> GMSEPYTWKSVVTGAGGGFVPGIIFNQTEPNLIYARTAIGGAYRWNQATSSWVSISDSVGWVDWNKNGVDALATDPIDPNKVYMATGTYTNHWDNNGQIMRSNDRGNTWQTTPLPFKVGGNMPGRSAGERLVIDPNKNNILYFGARSGNGLWKSIDSGVTWSKVTSFPNVGTYIQNPTLDYGNDLVGLSWITFDKSTGTLGNATQTIYVGVADTASSVYRSTDGGVTWTALAGQPTGFLPHHGELSSTGDLYITYSNGVGPYDGSKGEVWKYNKTSGAWTNISPTTGTDNWYGFGGLALDAQHPNTLMVSSLNAWWPDEVIFRSTNGGATWSRIWDWGNYPERTYKFSMDITAAPWLDHGTTSTSLDPSPKLGWMMGDLEIDPFNSNRMMYGTGATIYGSNNLTSWDTGGKVNISVMAKGVEETAVLGLISPPTGTSHLITALGDVSGFRHEDLSVAPTKFQTSPSWATTMSIDYAELSPSYMVRVGSADKEKTPSMKSIGISNDGGVNWYMPNSEPSNGTKTTVGHGQVAVSASGNSILWSTSDIGVYYSKTSGNSWTASAGLPAGAKIASDRVNPNKYYGFYAGTFYVSVDGGATFTATGASGFPTNNVAGLQPNEAQISMKAVPGIEGDIWFAGGNTVENKY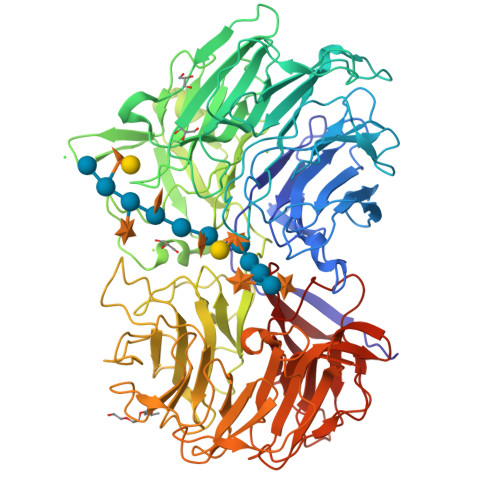GLWHSTNSGASFTKLTNVEEADLIGYGKAAPGQTYMSLYTVAKIDGVRGVFRSDDVGATWVRINDDAHQYAKINMAITGDPRIYGRVYLGTNGRGTLYADPV> MGSSHHHHHHSSGRENLYFQGHMNSPTSRPLRRDPLHNALVTTNVLVVLDQLEVAAEPTRRRLVQLLTSGEQTVNNLAAHFPASRSAISQHLRVLTEAGLVTPRKDGRFRYYRLDPQGLAQLRALFDSFWI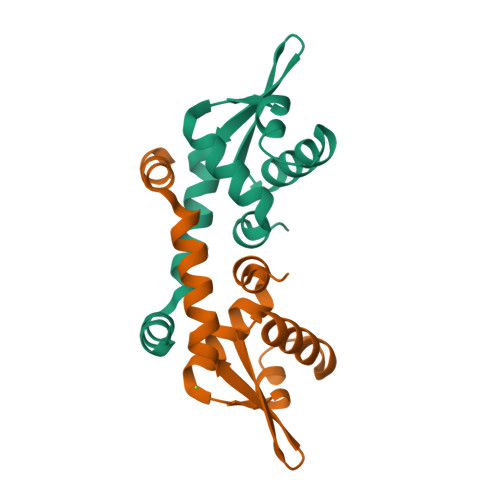DELDRLVADATEEAASKGDS The cellular fusion protein HAP2, which is structurally homologous to viral class II fusion proteins, drives gamete fusion across several eukaryotic kingdoms. HAP2/GCS1 is the first bona fide gamete fusion protein identified. The presence of HAP2 in organisms across the main branches of eukaryotes (Cole et al., 2014, Ebchuqin et al., 2014, Kawai-Toyooka et al., 2014, Steele and Dana, 2009) suggests that it is likely an ancestral gamete fusogen already present at the origin of eukaryotic life. The reported HAP2 structure displayed the three characteristic β sheet-rich domains of viral class II fusion proteins, organized around the central domain I. In the post-fusion form, domain I is a 10-stranded β sandwich with the inner A0B0I0H0G0 β sheet packing against the outer J0C0D0E0F0 β sheet.

Here, we report the X-ray structure of the C. reinhardtii HAP2 ectodomain derived from a different crystal form that resolves most of the regions that were missing in the previous structure. The complex with the single-chain variable fragment (scFv) of one of these antibodies resulted in crystals in the hexagonal space group P6322 diffracting to 2.6 Å resolution. In total, the new model contains 551 out of 573 residues, with a break of about 15 residues in the fg loop in domain II—a loop projecting laterally, perpendicular to the trimer axis and roughly midway between top and bottom. The three “fusion helices” are arranged into a horseshoe shape, exposing the non-polar residues toward the target membrane. αF1 is 9 aa long and exposes residues W173 and F177; ηF is only one turn and exposes F192 and W193, and αF2 is 7 aa long and exposes P196, L197, L200, and I201. Mutagenesis altering the non-polar character of the exposed residues in the fusion helices disrupted the ability of the HAP2 ectodomain to insert into liposomes. The 37-residue long C0D0 loop is completely resolved in the new structure, and displays a CLL motif with three parallel disulfide bonds. Although the new crystals did not entirely resolve the E0F0 loop, they showed density for its N-terminal six amino acids (aa) (sequence PTAPSP, downstream of strand E0) as well as its C-terminal 14 residues (271-APQFLSPPAPSTRE-285) preceding β strand F0, accounting in total for 40% of the loop. The new structure resolves the N-terminal 12 residues of the stem, showing that it is directed toward the tip of domain II of the adjacent “left” subunit in the trimer. The HAP2 stem fills a surface groove in the adjacent protomer, formed between the bc loop and the aefg β sheet of domain II. The packing between HAP2 trimers in the new crystals involves 2-fold symmetric head-to-head interactions along the 3-fold crystallographic axis.

> RSEVIASGRLEKCVVDGVTEELDCQEKVVVTLTVGNGQSLQTEALEFSLSCLNSPDGRCPCSCSAADPTCACRDLAAPLRVSLTKSPLWASYPLQYLSSFNWKPLEVILRPSNKVCKDGDWEDSPTCGWFSQGGVRVADSQGFCCECSSSQVWDDTFGSSKERTRANLDCDFWSDPLDILIGRKPVSAHCLTFDPQWYSGYELGAASLQFEIAITVEVPTAPSPTTATTSATPRTNNSSSANSTNSTNSPAPQFLSPPAPSTREVLHLGPSVPLASSASRLLSAKLLGDLAMYTQLPAISNQVLMVPQPPAAAAATGSPLDATLATNRSAWMLLDKTMLSMDGLACDKVGTGFSAFRYQPSGCGRAPQACLSGQLKDLWEADLARIADGRVPLYMITRFTGGSDTTLQSFSGGPLSFALPVTSHSQSLVTLSVAADGVRLVTNRSPGKITGAAVCRFAGTSCGGFEAVAARGYIYVNITNTGRLDSDYTLTVSNCSSNVRPIEARTLAVRAGSAASLDPPMELYVEDQAAAAARTCTVSLYDSVGAVTDSLTLSFYTNATQLVVKPSGGYNGGPFEDDDDK PLLs are natural lactonases endowed with promiscuous phosphotriesterase activity. The catalytic center contained two metal cations coordinated by four histidines, an aspartic acid and a carboxylated lysine residue. A structural analysis of SsoPox, a hyperthermostable counterpart of the PLL family from Sulfolobus solfataricus, has revealed that loop 7 is shorter in SsoPox than in PTEs; linking the active site to the loop 8, which forms a hydrophobic channel that accommodates AHLs aliphatic chain. Indeed, W263 is located at the start of loop 8, involved in the dimer interface of the enzyme and positions the lactone cycle of the substrate onto the bi-metallic catalytic center.

Co-crystallization assays with C10-HTL were performed using the same protocol but adding 4 µL of a 60 mM C10-HTL solution (in Ethyl acetate:DMSO; 1:1) to 120 µL of the protein solution. Crystals were first transferred to a cryoprotectant solution composed of the reservoir solution and 20% (v/v) glycerol, a 1/30 (v/v) ratio of a 60 mM C10 HTL solution was added to the cryo-protectant solution for co-crystallization trials. The diffraction data for W263F and W263I-C10 HTL crystals were collected at the Proxima-1 beam line (SOLEIL, Gif-sur-Yvette, France) using a PILATUS-6M detector. However, whereas detergent-induced flexibility has no effect on the lactonase activity, we isolated variants of W263 that exhibit increased lactonase activities (W263T/V/I). These variants exhibit dramatic improvement of their oxo-lactonase catalytic efficiencies (148-fold for variant W263T), while the activity for the best AHL substrate is compromised (3-oxo-C10 AHL; for the wild-type enzyme). Conversely, the LacSV group dramatically increases oxo-lactonase activity and 3-oxo-C12 AHLase activities, while the phosphotriesterase activity is mildly modulated and 3-oxo-C10 AHLase is decreased. The residues selected in the LacSV group (T, V, I) are overall smaller than those selected in the PteSV group (F, L, M) with the exception of isoleucine (I). Noteworthy, subtle changes, such as W263L or W263I, yield to a large tradeoff in catalytic activities.

>MRIPLVGKDSIESKDIGFTLIHEHLRVFSEAVRQQWPHLYNEDEEFRNAVNEVKRAMQFGVKTIVDPTVMGLGRDIRFMEKVVKATGINLVAGTGIYIYIDLPFYFLNRSIDEIADLFIHDIKEGIQGTLNKAGFVKIAADEPGITKDVEKVIRAAAIANKETKVPIITHSNAHNNTGLEQQRILTEEGVDPGKILIGHLGDTDNIDYIKKIADKGSFIGLDRYGLDLFLPVDKRNETTLRLIKDGYSDKIMISHDYCCTIDIGTAKPEYKPKLAPRWSITLIFEDTIPFLKRNGVNEEVIATIFKENPKKFFS[4x]> AASSLDELVALCKRRGFIFQSSEIYGGLQGVYDYGPLGVELKNNLKQAWWRRNVYERDDMEGLDASVLTHRLVLHYSGHEATFADPMVDNRITKKRYRLDHLLKEQPEEVLKRLYRAMEVEEENLHALVQAMMQAPERAGGAMTAAGVLDPASGEPGDWTPPR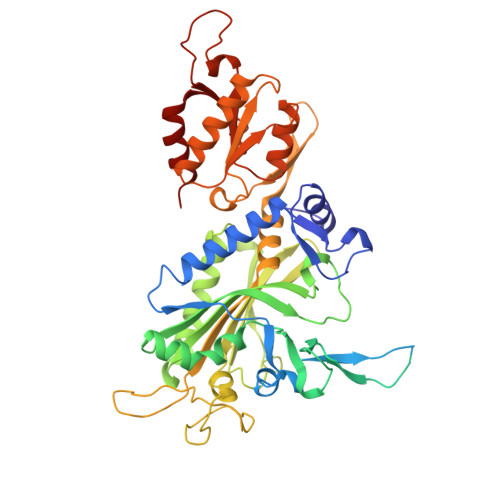YFNMMFQDLRGPRGGRGLLAYLRPETAQGIFVNFKNVLDATSRKLGFGIAQIGKAFRNEITPRNFIFRVREFEQMEIEYFVRPGEDEYWHRYWVEERLKWWQEMGLSRENLVPYQQPPESSAHYAKATVDILYRFPHGSLELEGIAQRTDFDLGSHTKDQEALGITARVLRNEHSTQRLAYRDPETGKWFVPYVIEPSAGVDRGVLALLAEAFTREELPNGEERIVLKLKPQLAPIKVAVIPLVKNRPEITEYAKRLKARLLALGLGRVLYEDTGNIGKAYRRHDEVGTPFAVTVDYDTIGQSKDGTTRLKDTVTVRDRDTMEQIRLHVDELEGFLRERLRW> MAISLATKAATDALKVNRAPVGVEPQEVHKWLQSFNWDFKENRTKYPTKYHMANETKEQFKVIAKEYARMEAAK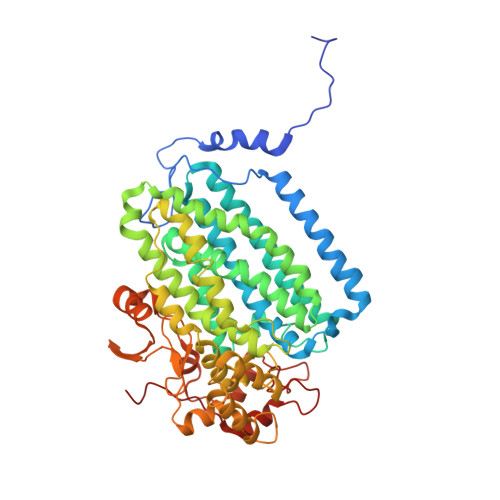DERQFGTLLDGLTRLGAGNKVHPRWGETMKVISNFLEVGEYNAIAASAMLWDSATAAEQKNGYLAQVLDEIRHTHQCAFINHYYSKHYHDPAGHNDARRTRAIGPLWKGMKRVFADGFISGDAVECSVNLQLVGEACFTNPLIVAVTEWASANGDEITPTVFLSVETDELRHMANGYQTVVSIANDPASAKFLNTDLNNAFWTQQKYFTPVLGYLFEYGSKFKVEPWVKTWNRWVYEDWGGIWIGRLGKYGVESPASLRDAKRDAYWAHHDLALAAYAMWPLGFARLALPDEEDQAWFEANYPGWADHYGKIFNEWKKLGYEDPKSGFIPYQWLLANGHDVYIDRVSQVPFIPSLAKGTGSLRVHEFNGKKHSLTDDWGERQWLIEPERYECHNVFEQYEGRELSEVIAEGHGVRSDGKTLIAQPHTRGDNLWTLEDIKRAGCVFPDPLAKF>[2x]MSSSAMPDVPAPLTNLQFKYTKIFINNEWHSSVSGKKFPVFNPATEEKLCEVEEGDKEDVDKAVKAARQAFQIGSPWRTMDASERGRLLNKLADLIERDRLLLATMEAMNGGKLFSNAYLMDLGGCIKTLRYCAGWADKIQGRTIPMDGNFFTYTRSEPVGVCGQIIPWNFPLL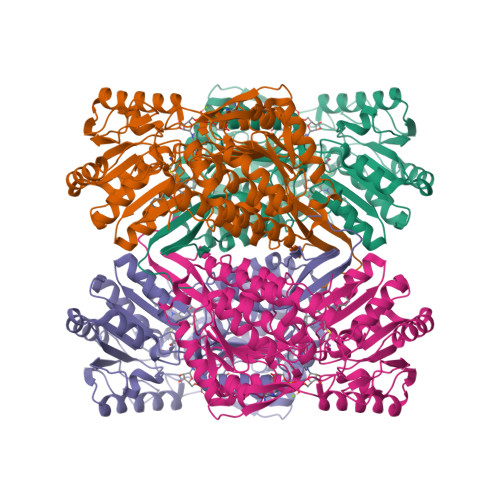MFLWKIGPALSCGNTVVVKPAEQTPLTALHMGSLIKEAGFPPGVVNIVPGYGPTAGAAISSHMDVDKVAFTGSTEVGKLIKEAAGKSNLKRVSLELGGKSPCIVFADADLDNAVEFAHQGVFYHQGQCCIAASRLFVEESIYDEFVRRSVERAKKYVLGNPLTPGVSQGPQIDKEQYEKILDLIESGKKEGAKLECGGGPWGNKGYFIQPTVFSDVTDDMRIAKEEIFGPVQQIMKFKSLDDVIKRANNTFYGLSAGIFTNDIDKAITVSSALQSGTVWVNCYSVVSAQCPFGGFKMSGNGRELGEYGFHEYTEVKTVTIKISQKNS> EPEPWFFKNLSRKDAERQLLAPGNTHGSFLIRESESTAGSFSLSVRDFDQNQGEVVKHYKIRNLDNGGFYISPRITFPGLHELVRHYT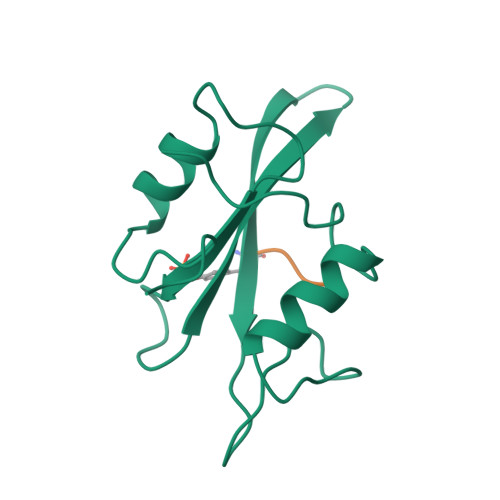NASDGLCTRLSRPCQT;> XYEEG>[2x]EPGENLKPVDAMQCFDCHTQIEDMHTVGKHATVNCVHCHDATEHVETASSRRMGERPVTRMDLEACATCHTAQFNSFVEVRHESHPRLEKATPTSRSPMFDKLIAGHGFAFEHAEPR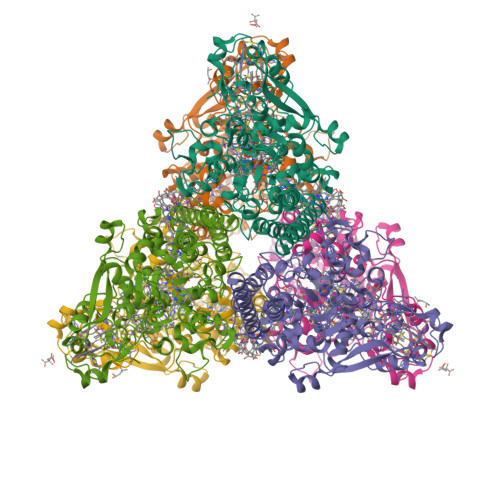SHAFMLVDHFVVDRAYGGRFQFKNWQKVTDGMGAVRGAWTVLTDADPESSDQRRFLSQTATAANPVCLNCKTQDHILDWAYMGDEHEAAKWSRTSEVVEFARDLNHPLNCFMCHDPHSAGPRVVRDGLINAVVDRGLGTYPHDPVKSEQQGMTKVTFQRGREDFRAIGLLDTADSNVMCAQCHVEYNCNPGYQLSDGSRVGMDDRRANHFFWANVFDYKEAAQEIDFFDFRHATTGAALPKLQHPEAETFWGSVHERNGVACADCHMPKVQLENGKVYTSHSQRTPRDMMGQACLNCHAEWTEDQALYAIDYIKNYTHGKIVKSEYWLAKMIDLFPVAKRAGVSEDVLNEARELHYDAHLYWEWWTAENSVGFHNPDQARESLMTSISKSKEAVSLLNDAIDAQVASR> DE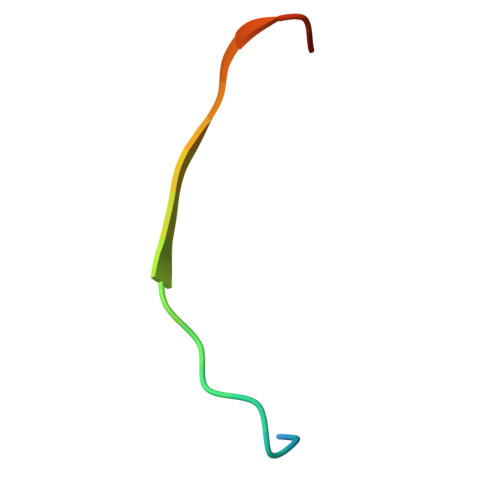QSGISQTVIVGPWGAKVS>[2x]MDSKQQCVKLNDGHFMPVLGFGTYAPPEVPRSKALEVTKLAIEAGFRHIDSAHLYNNEEQVGLAIRSKIADGSVKREDIFYTSKLWSTFHRPELVRPALENSLKKAQLDYVDLYLIHSPMSLKPGEELSPTDENGKVIFDIVDLCTTWEAMEKCKDAGLAKSIGVSNFNRRQLEMILNKPGLKYKPVCNQVECHPY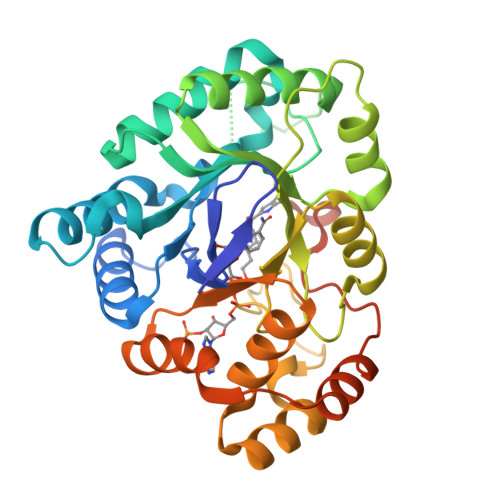FNRSKLLDFCKSKDIVLVAYSALGSQRDKRWVDPNSPVLLEDPVLCALAKKHKRTPALIALRYQLQRGVVVLAKSYNEQRIRQNVQVFEFQLTAEDMKAIDGLDRNLHYFNSDSFASHPNYPYSDEYLEHHHHHH>[3x]GAMATTKIRIFVPATNSPELRWELTLFALDVIRSPSAAESMKVGAAFTLISMYSERPGALIRSLLNDPDIEAVIIDVGSMVNGIPVMERRGDKAQEEMEGLMRILKTARDSSKGKTPFVDSRAYGLRITDMSTLVSAVITIEAQIWILIAKAVTAPDTAEESETRRWAKYVQQKRVNPFFALTQQWLTEMRNLLSQSLSVRKFMVEILIEVKKGGSAKGRAVEIISDIGNYVEETGMAGFFAT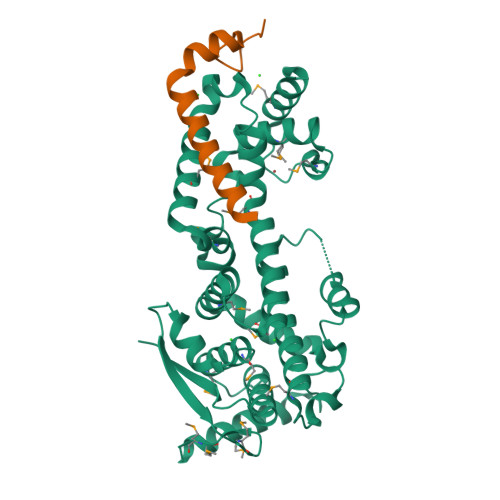IRFGLETRYPALALNEFQSDLNTIKSLMLLYREIGPRAPYMVLLEESIQTKFAPGGYPLLWSFAMGVATTIDRSMGALNINRGYLEPMYFRLGQKSARHHAGGIDQNMANRLG;>[3x]GAMDKLELVNDGLNIIDFIQKNQKEIQKTYGRSSIQQPSIKDQTKAWEDFLQ The LINC complex, consisting of interacting SUN and KASH proteins, mechanically couples nuclear contents to the cytoskeleton. The SUN protein has an N-terminal nuclear region, crosses the inner nuclear membrane, and then traverses the nuclear lumen (perinuclear space) to position its C-terminal SUN domain immediately below the outer nuclear membrane. SUN1 is essential for meiosis as its disruption in mice leads infertility owing to failure of chromosome synapsis. The luminal region of SUN proteins upstream of the SUN domain is thought to consist of a long trimeric coiled-coil that passes between nuclear membranes.

On the basis of conservation and secondary structure prediction, we identified a 40 amino-acid coiled-coil domain towards the beginning of human SUN1’s luminal region (amino-acids 362–401; herein referred to as α1), which was stable in solution following recombinant expression. We obtained crystals of SUN1 α1 that diffracted anisotropically to a maximum resolution limit of 2.1 Å, and solved its X-ray crystal structure by molecular replacement of ideal helical fragments using ARCIMBOLDO_LITE in ‘coiled-coil’ mode. This revealed a parallel trimeric coiled-coil of approximately 6 nm in length, in which the “a” and “d” heptad amino-acids are conserved across vertebrates. At the centre of the SUN1 α1 coiled-coil structure is a 376-CHHH-379 motif, in which the cysteine residues are at the “a” position of the heptad repeat and are oriented away from the coiled-coil axis. We observed additional electron density for one cysteine of the trimer, which points towards the coiled-coil axis, likely representing an oxidised cysteine residue. On the basis of the additional density, we modelled this as S-hydroperoxycysteine, as an alternative conformation of the reduced cysteine residue, which refined with relative occupancies of 0.62 and 0.38, respectively. The oxidised C376 residue is packed within the core of the structure, so likely provided additional stability to the coiled-coil, and may have assisted the formation of a robust crystal system suitable for X-ray diffraction. Further, it creates an asymmetry in the structure, explaining the lack of crystallographic three-fold symmetry, with the full trimer constituting the crystal’s asymmetric unit. The trimeric coiled-coil on the N-terminal side is formed by heptad amino-acids V365, V369 and L372, whilst the coiled-coil on the C-terminal side is formed by heptad residues L386, L390, L393, V397 and M400. Further, the crystal structure lacked bound zinc, but included a partially oxidised cysteine residue, which seemingly provided an alternative means for structural stabilisation.

>GSMSGVEQQVASLSGQCHHHGENLRELTTLLQKLQARVDQME[3x]>SFHQECSLQSCAQHQPYVVDDPCPIHFYSKWYIRVGARKSAPLIELCVDEVGSKSPIQYIDI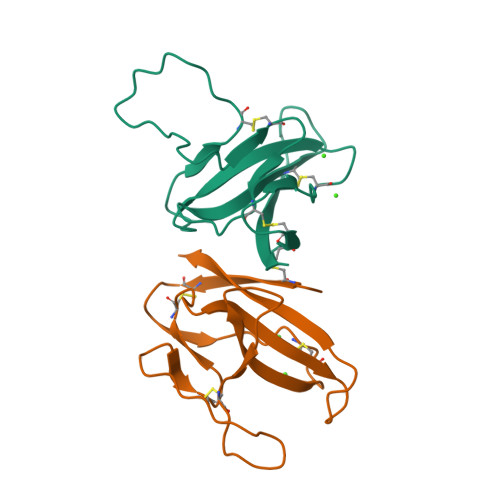GNYTVSCSPFTINCQEPKLGSLVVRCSFYEDFLEYHDVRVVLDFI[2x]Ribosomal protein S6 kinase 1 (S6K1) is a serine/threonine protein kinase that plays an important role in the PIK3/mTOR signaling pathway, and is implicated in diseases including diabetes, obesity, and cancer. All of the inhibitors bound to the ATP binding site, lying along the P-loop, while the activation loop stayed in the inactive form. The zinc-binding site is composed of the C–H–H–C residues, and is located in the middle of the activation loop.

The published S6K1-specific inhibitor, PF-4708671, was also used in this study. Recently, the structures of S6K1 complexed with PF-4708671 were published, with either the S6K1KD protein or the protein with the C-terminal extension including the hydrophobic motif (S6K1HM) and its derivatives. PF-4708671 has an ethyl group on the pyrimidine ring, which is accommodated in the hydrophobic pocket formed by Val105, Ala121, and Leu172, next to the hinge-binding site, while F108 and F109 have fewer hydrophobic interactions in these regions. The inhibitor interacts with the hinge region, and its pyrimidyl nitrogen atom forms a hydrogen bond with the amide nitrogen atom of Leu175. The ethyl group is located in the hydrophobic environment formed by Val105, Ala121, and Leu172. The trifluoromethyl group contacts the side chains of Leu125 and Lys123 and the main chain of Gly103. As compared with PF-4708671, the five inhibitors found in this study have lower potencies, in terms of the IC50 values ranging from two- to more than 40-fold. Ala134 and Lys135 form the N-terminal cap of helix αC in the complex structures with PF-4708671, F176, and F177, where the side chain of Asp136 interacts with the hydroxyl group of Tyr102 in the P-loop. In these S6K1KD structures, a strong electron density peak was observed in the Fourier difference maps and anomalous difference Fourier maps. This peak was assigned to zinc for the PF-4708671 complex.

> GSFTSSGSVNRGPEKIRPECFELLRVLGKGGYGKVFQVRKVTGANTGKIFAMKVLKKAMIVRNAKDTAHTKAERNILEEVKHPFIVDLIYAFQTGGKLYLILEYLSGGELFMQLEREGIFMEDTACFYLAEISMALGHLHQKGIIYRDLKPENIMLNHQGHVKLTDFGLCKESIHDGTVTHTFCGTIEYMAPEILMRSGHNRAVDWWSLGALMYDMLTGAPPFTGENRKKTIDKILKCKLNLPPYLTQEARDLLKKLLKRNAASRLGAGPGDAGEVQAHPFFRHINWEELLARKVEPPFKPLLQSEEDVSQFDSKFTRQTPVDSPDDST>[4x]SMTKTWTLKKHFVGYPTNSDFELKTSELPPLKNGEVL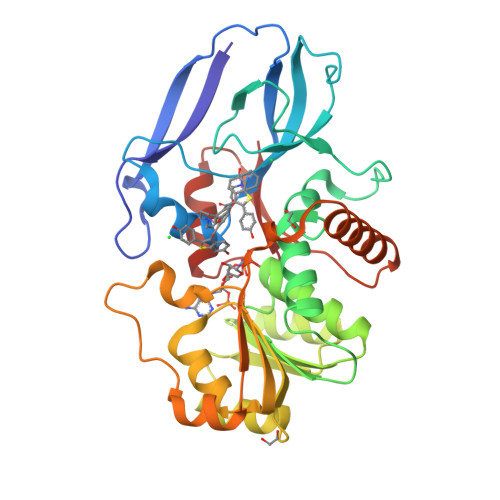LEALFLTVDPYMRVAAKRLKEGDTMMGQQVAKVVESKNVALPKGTIVLASPGWTTHSISDGKDLEKLLTEWPDTIPLSLALGTVGMPGLTAYFGLLEICGVKGGETVMVNAAAGAVGSVVGQIAKLKGCKVVGAVGSDEKVAYLQKLGFDVVFNYKTVESLEETLKKASPDGYDCYFDNVGGEFSNTVIGQMKKFGRIAICGAISTYNRTGPLPPGPPPEIVIYQELRMEAFVVYRWQGDARQKALKDLLKWVLEGKIQYKEYIIEGFENMPAAFMGMLKGDNLGKTIVKA>[8x]KVKVW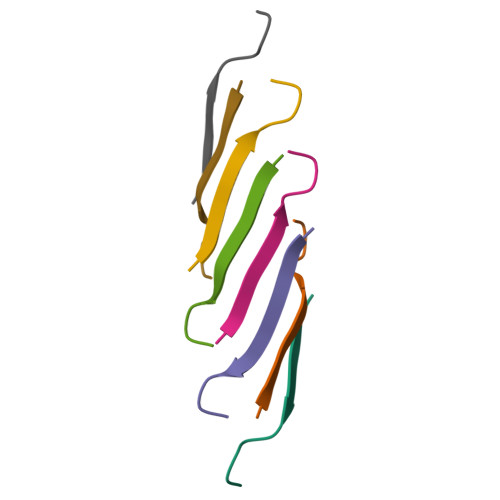GSIKGL> MAVEKTNSSSSLAEVIDRILDKGIVIDAWVRVSLVGIELLAI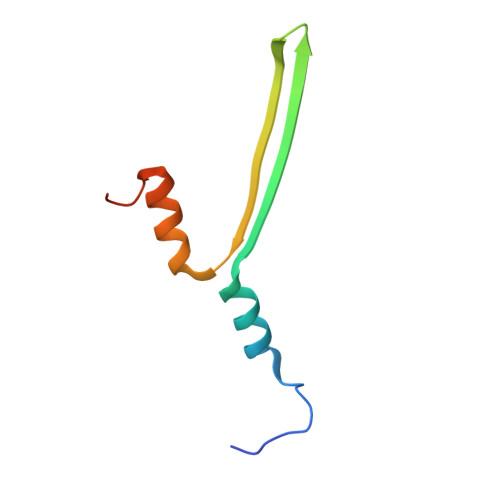EARIVIASVETYLKYAEAVGLTQSAAVPA>[4x]MSEQQVQELEKKWYALQVEPGKENEAKENLLKVLELEGLKDLVDEVIVPAEEKVVIRAQGKEKYRLSLKGNARDISVLGKKGV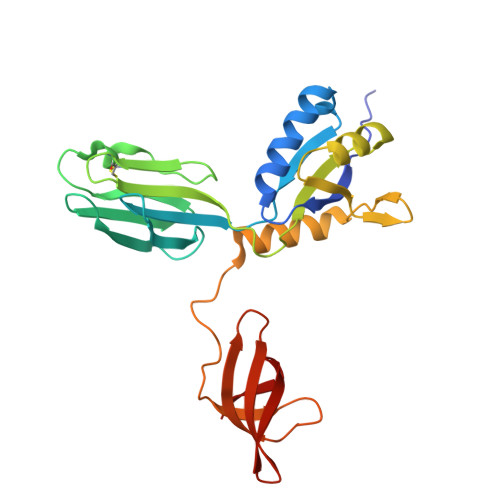TTFRIENGEVKVVESVEGDTCVNAPPISKPGQKITCKENKTEAKIVLDNKIFPGYILIKAHMNDKLLMAIEKTPHVFRPVMVGGKPVPLKEEEVQNILNQIKRGVKPSKVEFEKGDQVRVIEGPFMNFTGTVEEVHPEKRKLTVMISIFGRMTPVELDFDQVEKI> MQAVTRFFRHLITLTAVALLAAFLDTVNAAKDTAAGHVTTPCTEILFDLTLAKHYENQIQAAESALNRNYAAIRSWTLLEAMSSDGNRQNAYTGLIAYGIQITVNAEQELQGPKQTKLRAAAALRHRAANLSAALQIQAAQQATLTKPTAGGAQTPFSGATGTCKYEGITATAGEQSCKYSTEDEEKINAAHMNPEVMTQITTIGDKYLTTITLDAIAGSKGNPTQSSATYAEQDCQ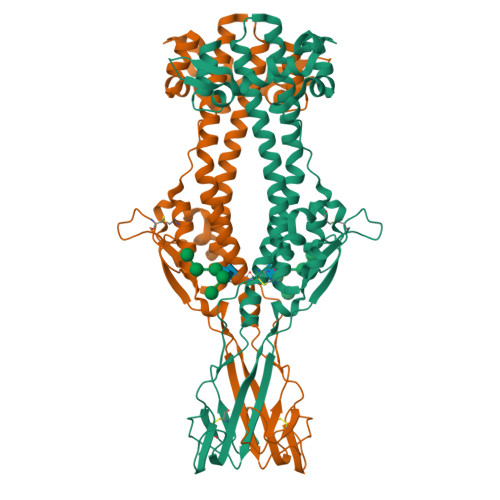DGGNPGPNFGGANALGLQVTKLGTKATTEKTNLYTAGGTECEHQPGNGPQKTKQRLAYLVCEANKAAIITPTDLQTLTLDALISAPEMAAIGDALLTDEPATEKEYSSAQHTQIQQLLKKAYGQTNEQFQKNFIKPLAAQTVKFKIGGAEVSNTVAALMSSPNSGLALAYHKGKNKLQHQVKPDTPLVESKKGSECQVIEDKEKCKTTYGCELKGDKCVVKMTTKGEVTGTQNTTGSNSFVIKKAPLLLAFLLF1-[5-tert-butyl-2-(4-methylphenyl)-1,2-dihydro-3H-pyrazol-3-ylidene]-3-{3-[(pyridin-3-yloxy)methyl]-1H-pyrazol-5-yl}urea 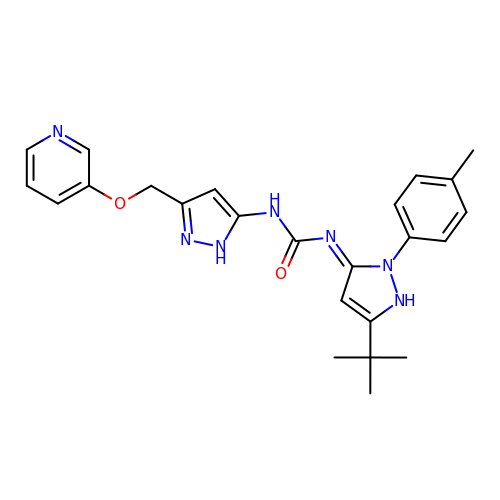| C24 H27 N7 O2 | OGYYVRWSDKOCHJ-HPNDGRJYSA-N> QDADKLPHTKVTLVAPPQVHPHEQATKSGPKVVEFTMTIEEKKMVIDDKGTTLQAMTFNGSMPGPTLVVHEGDYVQLTLVNPATNAMPHNVDFHGATGALGGAKLTNVNPGEQATLRFKADRSGTFVYHCAPEGMVPWHVVSGQSGTLMVLPRDGLKDPEGKPLHYDRAYTIGEFDLYIPKGPDGKYKDYATLAESYGDTVQVMRTL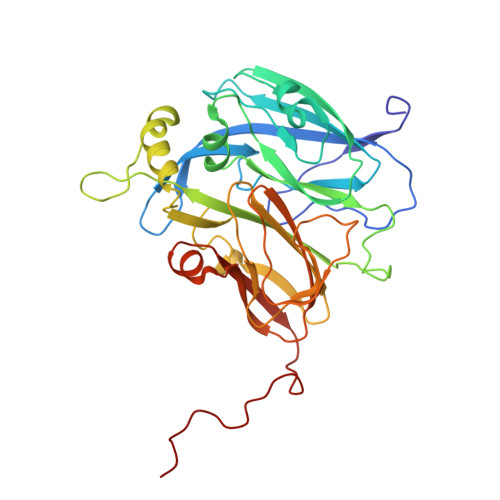TPSHIVFNGKVGALTGANALTAKVGETVLLIHSQANRDTRPHLIGGHGDWVWETGKFANPPQRDLETWFIRGGSAGAALYTFKQPGVYAYLNHNLIEAFELGAAGHIKVEGKWNDDLMKQIKAPAPIPR> EEPPKEKLHTLEEFSYEFFRAPEKDMVSMAVLPLARARGHLWAYSCEPLRQPLLKRVHANVDLWDIACQIFVAILRYMGDYPSRQAWPTLELTDQIFTLALQHPALQDEVYCQILKQLTHNSNRHSEERGWQLLWLCTGLFPPSKGLLPHAQKFIDTRRGKLLAPDCSRRIQKVLRTGPRKQPPHQVEVEAAEQNVSRICHKIYFPNDTSEMLEVVANTRVRDVCDSIATRLQLASWEGCSLFIKISDKVISQKEGDFFFDSLREVSDWVKKNKPQKEGAPVTLPYQVYFMRKLWLNISPGKDVNADTILHYHQELPKYLRGFHKCSREDAIHLAGLIYKAQFNNDRSQLASVPKILRELVPENLTRLMSSEEWKKSILLAYDKHKDKTVEEAKVAFLKWICRWPTFGSAFFEVKQTSEPSYPDVILIAINRHGVLLIHPKTKDLLTTYPFTKISSWSSGSTYFHMALGSLGRGSRLLCETSLGYKMDDLLTSYVQQLLSAMNKQRGSKAPALAST;> QDFRKYEEGFDPYSMFTPEQIMGKDVRLLRIKKEGSLDLALEGGVDSPIGKVVVSAVYERGAAERHGGIVKGDEIMAINGKIVTDYTLAEAEAALQKAWNQGGDW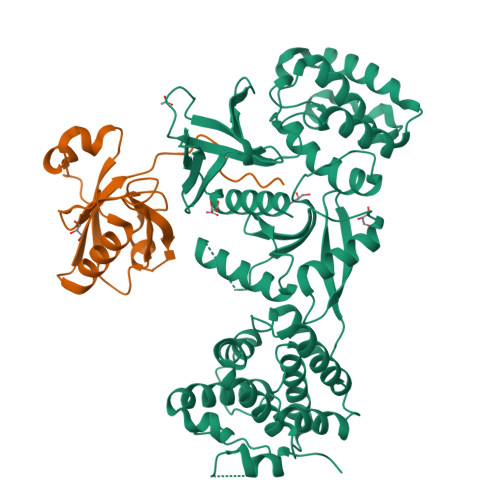IDLVVAVCPPKEYDDELTFF>[6x]PCCELITNISIPDDKAQNTLSEIEDAISNILGKPVAYIMSNYDYQKNLRFSGSNEGYCFVRLTSIGGINRSNNSLLADKITKILSNHLSVKPRRVYIEFRDCSAQNFAFSGSLF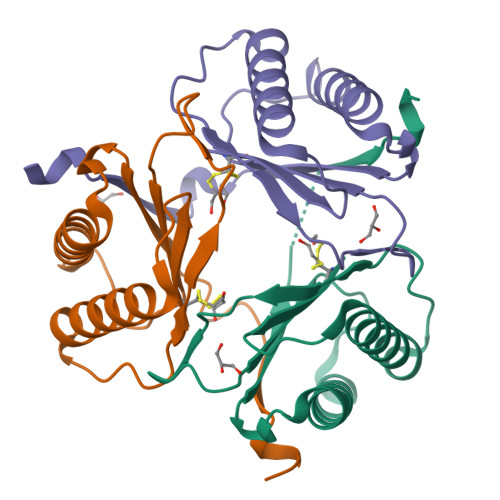GGSRSHHHHHH>GHMGAFTGKTVLILGGSRGIGAAIVRRFVTDGANVRFTYAGSKDAAKRLAQETGATAVFTDSADRDAVIDVVRKSGALDILVVNAGIGVFGEALELNADDIDRLFKINIHAPYHASVEAARQMPEGGRILIIGSVNGDRMPVAGMAAYAASKSALQGMARGLARDFGPRGITINVVQPGPIDTDANPANGPMRDMLHSLMAIKRHGQPEEVAGMVAWLAGPEASFVTGAMHTIDGAFGAG[2x]

The gene bdcA (also referred to as yjgI) was previously identified as a regulator of biofilm dispersal. BdcA expression decreases extracellular polysaccharide (EPS) production, cell length and aggregation while simultaneously increasing extracellular DNA production and motility. The structure of BdcA reveals that it is a member of the short-chain dehydrogenase/reductase family of enzymes. Using two complementary binding assays, we show that BdcA binds specifically to NADPH, and thus is highly likely its endogenous cofactor.

Here, we describe the crystal structure of BdcA at 2.05 Å, where we show that BdcA is a member of the short-chain dehydrogenase/reductase family. The SDR active site consists of a conserved catalytic triad (Ser-Tyr-Lys), which is C-terminal to the cofactor binding motif, Gly-X3-Gly-X-Gly. In contrast, NADP(H)-specific enzymes contain a basic residue within the glycine-rich motif immediately preceding the second conserved glycine, and/or in the loop after the second β-strand. These residue(s) are responsible for binding the 2′-phosphate. Furthermore, using isothermal titration calorimetry (ITC) and thermal stabilization assays, we identified the biologically relevant cofactor of BdcA to be NADPH. Previously, BdcA was hypothesized to suppress biofilm formation by binding and quenching the secondary messenger c-di-GMP. However, we were unable to show binding of c-di-GMP to BdcA using both DSF and ITC, excluding the possibility of a direct interaction. Furthermore, BdcA does not contain any of the well-known c-di-GMP binding motifs present in other proteins (GGDEF, EAL, HD-GYP). Thus, our data suggests that BdcA most likely influences biofilm dispersal by regulating a process that affects a c-di-GMP related pathway. Furthermore, because of its demonstrated role in biofilm dispersal, BdcA also represents an attractive target for dismantling biofilms.>[4x]HHHHHHFNLPPGNYKKPKLLYCSNGGHFLRILPDGTVDGTRDRSDQHIQFQLSAESVGEVYIKSTETGQYLAMDTDGLVY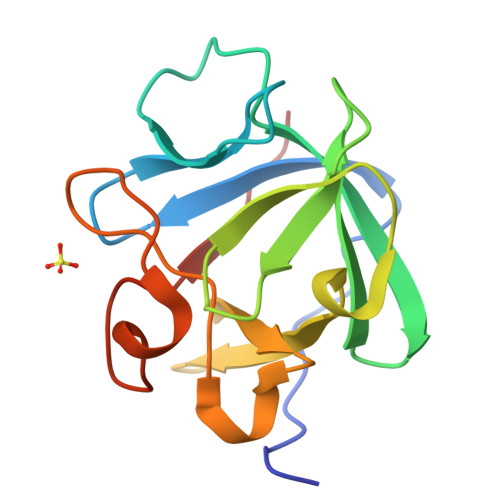GSQTPNEECLFLERLEENHYNTYISKKHAEKNWFLGLKKNGSCKRGPRTHYGQKAILFLPLPVSSD> MDQAVQEDFFTRLQTIIDSRGKKTVNQQSLISTLEELLTVAEKPYEFIMAYLTLIPSRFDASANLSYQPIDQWKSSFNDISKLLSILDQTIDTYQVNEFADPIDFIEDEPKEDSDGVKRILGSIFSFVERLDDEFMKSLLNIDPHSSDYLIRLRDEQSIYNLILRTQLYFEATLKDEHDLERALTRPFVKRLDHIYYKSENLIKIMETAAWNIIPAQFKSKFTSKDQLDSADYVDNLIDGLSTILSKQNNIAVQKRAILYNIYYTALNKDFQTAKDMLLTSQVQTNINQFDSSLQILFNRVVVQLGLSAFKLCLIEECHQILNDLLSSSHLREILGQQSLHRISLNSSNNASADERARQCLPYHQHINLDLIDVVFLTCSLLIEIPRMTAFYSGIKVKRIPYSPKSIRRSLEHYDKLSFQGPPETLRDYVLFAAKSMQKGNWRDSVKYLREIKSWALLPNMETVLNSLTERVQVESLKTYFFSFKRFYSSFSVAK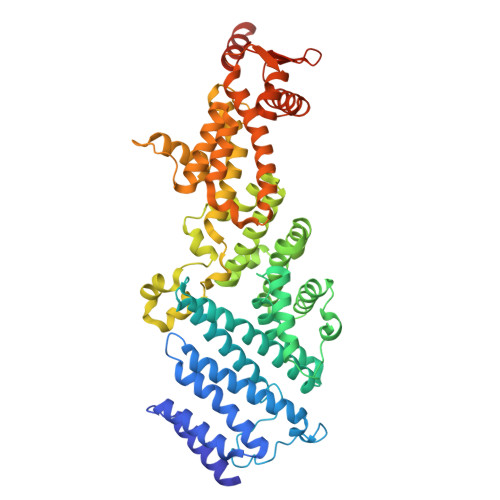LAELFDLPENKVVEVLQSVIAELEIPAKLNDEKTIFVVEKGDEITKLEEAMVKLNKEYKIAKERLNPPSNRR> MSSKPTDRGQQYKDGKFTQPFSLVNQPDAVGAPINAGDFAEQINHIRNSSPRLYGNQSNVYNAVQEWLRAGGDTRNMRQFGIDAWQMEGADNYGNVQFTGYYTPVIQARHTRQGEFQYPIYRMPPKRGRLSSRAEIYAGALSDKYILAYSNSLMDNFIMDVQGSGYIDFGDGSPLNFFSYAGKNGHAYRSIGKVIIDRGEVKKEDMSMQAIRHW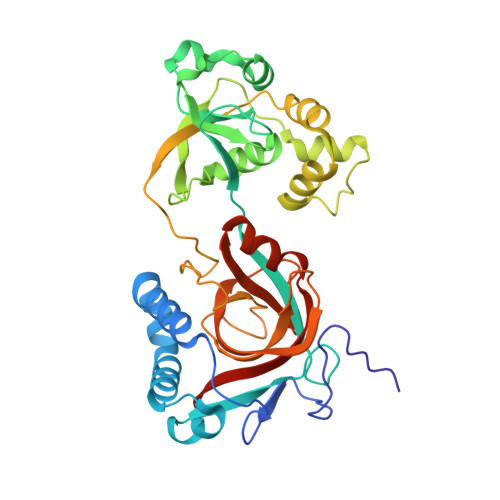GETHSEAEVRELLEQNPSFVFFKPQSFAPVKGASAVPLVGRASVASDRSIIPPGTTLLAEVPLLDNNGKFNGQYELRLMVALDVGGAIKGQHFAIYQGIGPEAGHRAGWYNHYGRVWVLKTAPGAGNVFSG> GSKKPRTPPVTLEAARDNDFAFDW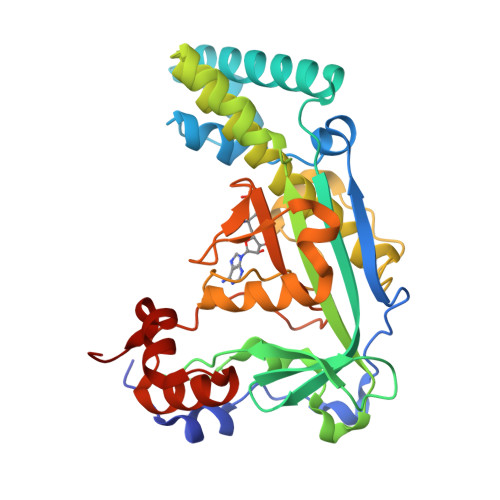QAYTPPVAHRLGVQEVEASIETLRNYIDWTPFFMTWSLAGKYPRILEDEVVGVEAQRLFKDANDMLDKLSAEKTLNPRGVVGLFPANRVGDDIEIYRDETRTHVINVSHHLRQQTEKTGFANYCLADFVAPKLSGKADYIGAFAVTGGLEEDALADAFEAQHDDYNKIMVKALADRLAEAFAEYLHERVRKVYWGYAPNENLSNEELIRENYQGIRPAPGYPACPEHTEKATIWELLEVEKHTGMKLTESFAMWPGASVSGWYFSHPDSKYYAVAQIQRDQVEDYARRKGMSVTEVERWLAPNLGYDAD> MHKSAFQALQGDIPTYEVNSSDEQDSDQDEEDVE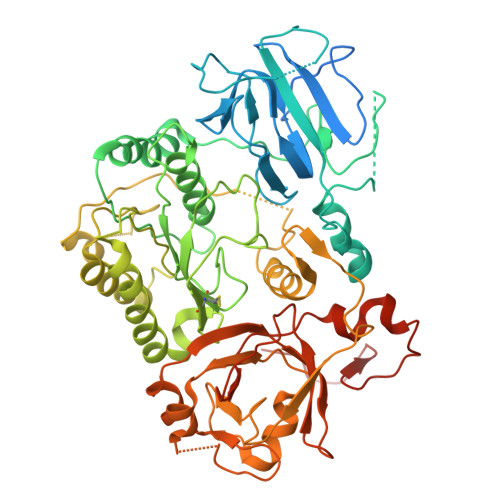QPSEPMHRLVSAPAASIHIEESKYISSNFSFDDDNTIYGHDYVIFGLKSNQNLIVKGQFVLEIQRGAIDINGVIYHSGVEPMKFINPSSSSIPLIQATQVLNSSLLENKESQENQHLFTPGYKSVIKLTNLDTHLESIGRVCPLFKNLFWQFDNFFAEDSLRLLDQYELAFSDYTFYPITKPDNTVSVIKHKNWMDVIKSLTELYSNDQSIKVIVIGGKNSGKSTFLRLLVQHMLSPTLQQLPINFMDLDPGQPEYSGTDCISLSKISEVQHGNHLSLTSTDSTQCHYVGFNSPKDQPTRYNLLVEQLVRSYESDGELKHESLLINTPGWIKGYGLELTRTLIERVKPTHVIYLNSGTLGVDIDIPKGTNLIPLQGSFNHSGSRYSSSQLRLLKTMAYFHKIDDFKFDFQPLLFSPPIQVSYGVSTGISALTHLKETGIGMDHLERSIEATIVGIFKVKRDHLEECELFNKGQLPLLPYKEFIKLSTEFFRLALVHSIDQEKKIMNLYIPQFRTLDLTKEAIIMVRGNTDLPIWEIASNEIVKRFKRQLPYITFEKGSSLEKKWKVRKNVQRRGQM>[2x]GADDVVD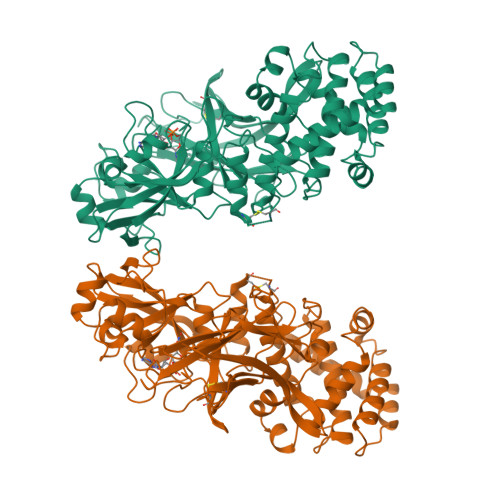SSKSFVMENFSSYHGTKPGYVDSIQKGIQKPKSGTQGNYDDDWKGFYSTDNKYDAAGYSVDNENPLSGKAGGVVKVTYPGLTKVLALKVDNAETIKKELGLSLTEPLMEQVGTEEFIKRFGDGASRVVLSLPFAEGSSSVEYINNWEQAKALSVELEINFETRGKRGQDAMYEYMAQACAGNRVRRSVGSSLSCINLDWDVIRDKTKTKIESLKEHGPIKNKMSESPNKTVSEEKAKQYLEEFHQTALEHPELSELKTVTGTNPVFAGANYAAWAVNVAQVIDSETADNLEKTTAALSILPGIGSVMGIADGAVHHNTEEIVAQSIALSSLMVAQAIPLVGELVDIGFAAYNFVESIINLFQVVHNSYNRPAYSPGHKTQPFLHDGYAVSWNTVEDSIIRTGFQGESGHDIKITAENTPLPIAGVLLPTIPGKLDVNKSKTHISVNGRKIRMRCRAIDGDVTFCRPKSPVYVGNGVHANLHVAFHRSSSEKIHSNEISSDSIGVLGYQKTVDHTKVNSKLSLFFEIKS> GAMVMINKENLSSQAKLWNFIYGFADSLVLKSAVQLDLANIIHNHGSPMTLSELSLHLPSQPVNQDALYRVLRYLVHMKLFTKSSIDGELRYGLAPPAKFLVKGWDKCMLGAILTITDKDFMAPWHYLKEGILNDGSTSTAFEKALGTNIWDYMAEHPEKNQLFNEGMANDTRLIMSALVKECSSMFDGITTIVDVGGGTGTAVRNIAKAFPHIKCTVYDLPHVIADSPGYTEINSIQGDMFKYIPNADAIMMKCILHDWDDKECIEILKRCKDAVPRDGGKVIIIDIILDVKSEHPYTKMRLTLDLDMMLNTGGKERTEEEWKKLIHDAGY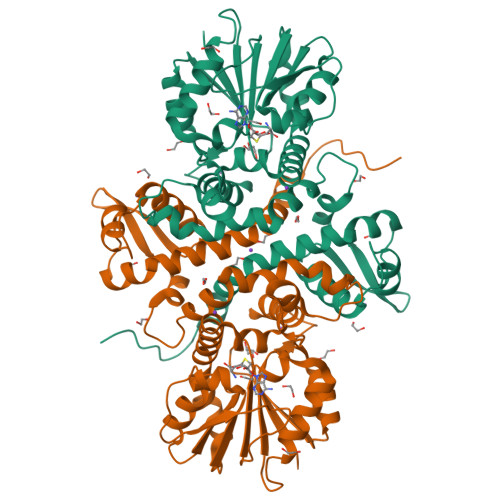KGYKITHISAVQSVIEAYPY>[3x]MNSICSLYCLFRRVMPYSSEILSSTVYRPPFLATSGLFFTRDHYKFIIMNQQQINPAQRSLRPRAQSAPSRSARRRRNRRRRNPSTPAGTVALQPSRITRRVVSNLARRPLTITTAGLAWLRQYLNPMGPSTSSVSGFPDGSAVTTCIADYTNTFNISFPPREAIYCTGSNSDEKPVMLDAATYAKIDAWTKSDITLCILALPMLRNVVMIRLYASTPTAFTLSEGVPNFVQRFPNWSAFTTEGKVLNNGDSPGYIQSFVYLPNVDKHLSAARGFRLLSRGLTGIYTAPSLETQGFVTA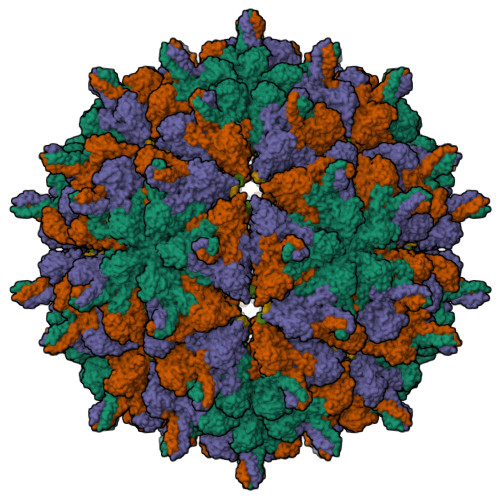CQYLAEGALQTQTVGNDFVQSVEVNADKTVKNVNGKRLHYSGPPKFVFPLEGDNCAPSSLVETYHQAYQARAVDGFYMPILSSSRDNPFISPKPQPIAVFNRWYYRGCLDPVPASKVADGPSQYYYDLNVADDVAPLYNTGVVWMEGISSKFSLKLKTRTVIQYIPTSGSVLANFTRHEPTYDQVALDAADRIRNMMPHAYPAAYNDWGWLGDLLDSTLSMLPGIGTAYRFAKPLIKPAWNWLGGKVSDFFGNPVSRDGDIYFDAK> MTVDFLSMVKYTPLFISGLIMTLKLTFLAVTIGVLMGLFIALMKMSSIKPIKLVASSYIEVIRGTPLLVQLLLIYNGLMQFGMNIPAFTAGVSALAINSS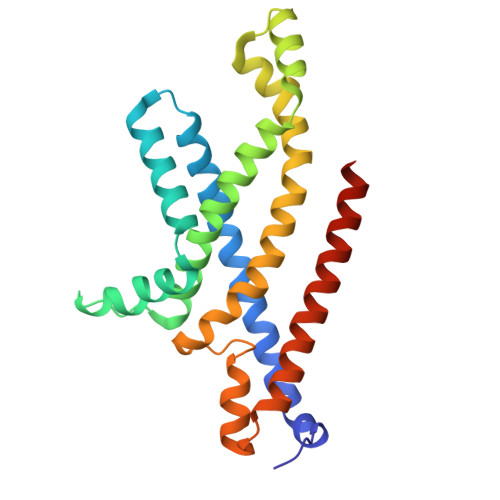AYVAEIIRAGIQAVDPGQNEAARSLGMTHAMAMRYVIIPQAIKNILPALGNEFIVMLKESAIVSVIGFADLTRQADIIQSVTYRYFEPYIIIAAIYFVMTLTFSKLLSLFERRLRAGDIR> UGCUCCUAGXACGAGAGGACCGGAG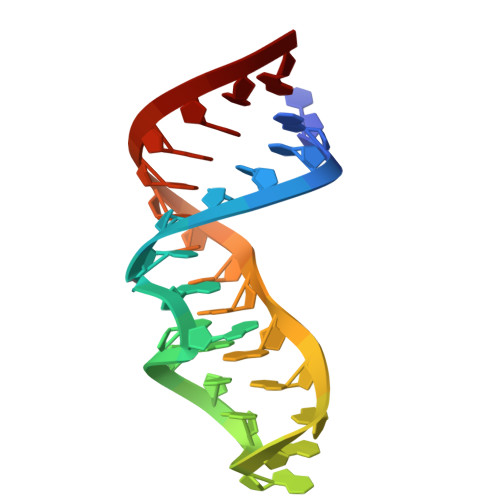UG>[2x]MADETIAIVDADATAETRSLLSYLDGVRGEGILFGHHGTTSSGLTTGPTDGTTSDVKNVTGDFPAVFGWSTSIIEGNQRPGLAENTRDENIALFADYIRKADAIGGVNTVGAGVENFVTGGSFYDTSGDTLRAVLPGGSHHAELVAYLDDIAELADASRRDDGTLIPIVFRPWHEN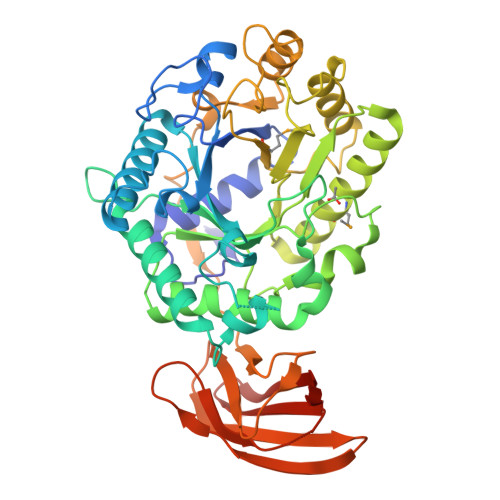AGSWFWWGAAYGSPGEYQELYRFTVEYLRDVKGVSNFLYAWGPGGGFGGNRDVYLRTYPGDAFVDVLGLDTYDSTGSDAFLAGLVADLRMIAEIADEKGKVSAFTRFGVSGGVGTNGSSPAQWFTKVLAAIKADPVASRNAYMETGENADAGQHFVPVPGDALLEDFQAYAADPFTLFASEVTGAFDRTVAAAPAQPVVHIASPADGARVASAPTTVRVRVGGTDVQSVTVEVAQGGTVVDTLDLAYDGALWWTAPWSPTSAQLDNSTYTVTATATTAAGTLDVTNEVAAALEHHHHHH> MYILDKIGLNIEILESLSYESKLGMSFKRTLSHFNKEEVLKEIELINNWYFSLEIIDDLPLDSRIKSVSSAKMKFERYYPNATYNRVFNDILGFRVICKSYDEVLELEKEDKIRVVDMSRGKSNDDGFRGIHVYYQRDNHHYP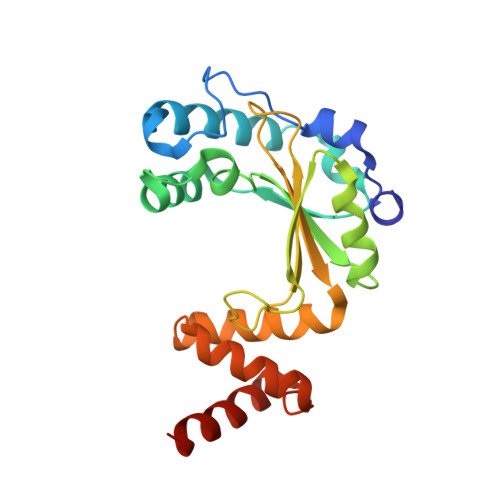IEIQFNTYYDRQLNDWLHDKFYKRGYDSSCGQLLRKYYENGKIKSAEELEEVLEDVLYHCKKI> MGSTHHHHHHSSGRENLYFQGHMEEEMQRHIKLTPSQTTPVVLVVGDPGRVDKVKMLCDSYVDLAYNREYKSVECTYKGQKFLCVSHGVGSAGCAICFEELMNNGAKVI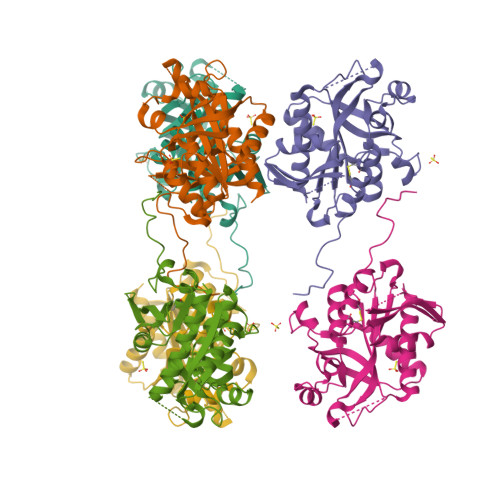IRAGSCGSLQPTQMKRGDICICNAAVREDRVSHLMIYSDFPAVADFEVYDTLNKVAQELEVPVFNGISLSSDLYYPHKIIPTRLEDYSKANVAVVEMEVATLMVMGTLRKVKTGGIFIVDGCPLKWDEGDFDNNLVPEKLENMIKISLETCARLAKKY> MKKGTASEEELKKLYDPNTFYEHGDNPAFKQFMNIAVENLREGKLTDHRTYVVDTYKKWMYARNWDDFLQRDCKAIT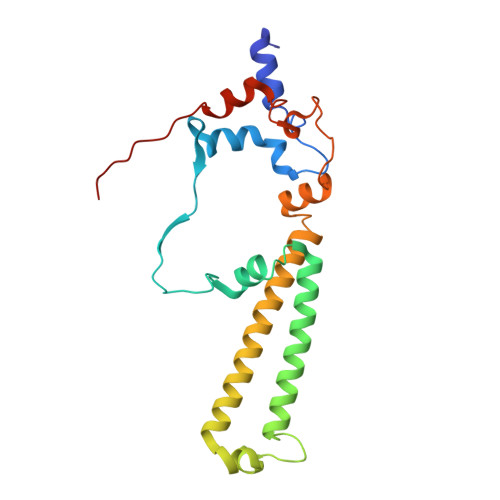FPRAFALWIVGTLGMATASKWCRQILPVGSHGITKISQTQFFHQFGPLGTLGAVGFYGLTAYLYYKTTIFTVKKFYSHCILQEREWIFEQERQNPGYGEYFFKDVPLSAEEHFNDLARGEMAKKKFEKPNHEF> SSITKDMKGFKVVEVGLA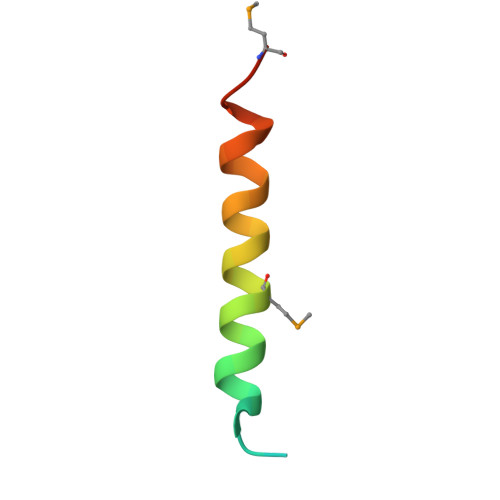MNTKKQIGDFFKNLNMAK>GSHMDKIRILWVDDEIDLLKPHILFLEKKNYEVTTSNNGLDAIALFEEENFDIVFLDENMPGMSGLETLSEMKEKKSAIPMIMITKSEEEYIMEEAIGSKIADYLIKPVNPNQILLSLKKNLDDSRLITEKTTLDYQKEFRKISMELAMVNSYEDWVELYKKLLFWELKLEDINDQAMIEILESQKVEANSQFGKYIERNYEDWFAPKADKPIQSHNLFKELVVPEIKKKDKPILFVVIDNLRYDQWKSFETVISNYYKLEKEVPYFSILPTAVQYARNAIFSGLMPLDMEKQFPQYWKNDVEDGGKNLYEAEFLSAQIKRLGLNIKEDYFKITNYAGGKKLAENFKALKGNDLVTVVYNFVDMLSHAKTEMEVVKELASDDKAYRSLTLSWFKNSPLLEIIQQAQLLGFKLILTTDHGTINVKNPSKVVGDKNTSLNLRYKTGRSLTYEQKDVYVVKEPKTIGLPAINMSSSFIFAKNDFFLAYVNNYNHYVSYYKNTYQHGGISLEEMIIPFLVFNPK[2x]

Here, we report on the structural determination of PorX, a noncanonical RR that comprises a classic REC domain and an additional enzymatic effector domain that exhibits phosphodiesterase activity. Our crystal structures reveal that the PorXFJ adopts a two-domain dimeric fold with a classical RR receiver domain's fold and a unique alkaline phosphatase superfamily (APS) domain connected by a helical linker region. Each PorXFJ monomer adopts a two-lobed fold containing an N-terminal receiver (REC) domain (residues 1–120), followed by a three-helix bundle (THB) domain (residues 121–209) and a C-terminal APS domain (residues 210–517). All PorXFJ dimers adopt an intertwined assembly, where each monomer is symmetrically wrapped around the other monomer, forming an overall “X”-like shape.

Additional support to the link between metal coordination and residues 358–369 conformation is provided by the T271V APS catalytically inactive mutant structure. In the T271V structure, a density corresponding to a divalent cation could only be observed in Zn1 site (coordinated by Asp360, His364, and His499) and not in the Zn2 site (coordinated by Thr271, Asp237, Asp414, and His415), while residues 358–369 of both monomers adopted a helical conformation instead of the helical-extended coil dyad observed in the same primitive orthorhombic crystal form of the wild type. Moreover, ICP-MS measurements revealed that the T271V mutant had a reduced ability to bind zinc with only 1.22 ions per monomer, instead of two seen by the wild type. Using the REC domain's phosphorylation-null mutant (D54A), the APS domain's catalytically inactive mutant (T271V) and their double mutant (D54A/T271V), we confirmed that these residues can specifically undergo phosphorylation in PorXFJ. Mutating the catalytic residues T271V, the metal-coordinating residues D360A/H364A, and the APS dimerization interface residues S384A/S388E, abolished the observed phosphodiesterase activity against bis-pNPP. For example, the catalytically inactive T271V variant exhibited a mixed population of both monomers and dimers, while the zinc coordination D360A/H364A double mutant remained mostly monomeric upon incubation with zinc. However, our attempts to co-crystalize the catalytically inactive T271V variant of PorXFJ with pGpG did not reveal the corresponding density in the APS catalytic site.> MIDLIVSQGRVADRAAWMIEGAARTARALEERYGLKGHYVGEPAPHADDDWSVALPQARETLVAVREAATESIKGDNLTVLVNNTHSVSLATLPVVAREHPDAVVLYIDGHGDFNTPETTDTGYLGGMVLSGACGLWDSGHGAGLRPEQAVLVGSRDIDEGERELIRKAGVRVIPPGEATAQAVLDAVKDAPVWISIDWDVLEPGSIPADYTVP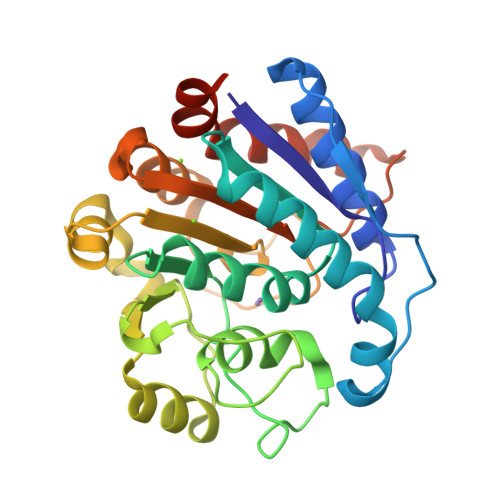DGMLPAQIRAVFEAIPAERLIGVELAELNAPADSERAEQAVAVILDMVAPAFDAAAARPLEHHHHHH> GSSHHHHHHSSGENLYFQHMASWD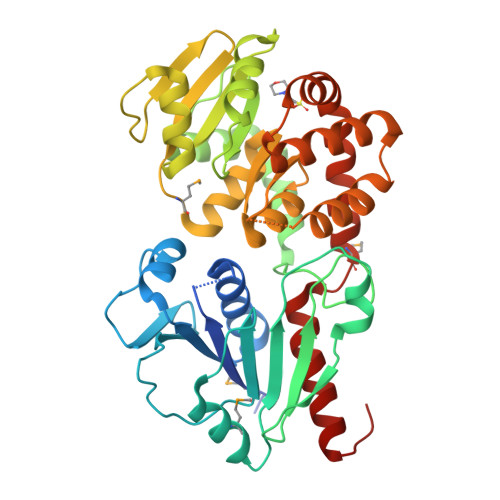IFCSVVDNYGDIGVTWRLARQLAAEHGQAVRLWVDEPQAFARICPRADPVAHVQCLDGVEVRAWGRPWAPVAAADVVIEAFACELPEAHRQAMRERKRPSLWLNLEYLSAEEWIGSCHALPSLQACGLSKYFFFPGFREPSGGLLREAGLLERRRRFQASVSAQDEFLASLGVRRKVGERLISLFAYENPALPGWLEQLRDARQPSLLLVPEGRVLADVADWLRVATLAVGDVHVRDALRVQVLPFMAQDDYDRLLWCCDLNAVRGEDSFVRAQWAGRPLLWHIYRQEEETHLAKLEAFLELYCAGLPADLAENLRTFWLAWNAGGGLAGAWEGLERQLPEWRREAQRWADEQGMRPDLAARLVQFYADWLLEHHHHHH The hetero-trimeric Sec protein-conducting channel translocates integral inner membrane proteins and secretory proteins into or across the membrane. The SecYEG core-translocon forms a central pore through which hydrophilic polypeptides are transported, otherwise closed by a girdle of hydrophobic residues and a short helix (plug)8. YidC is required to facilitate this passage from the lateral gate and for the subsequent folding and assembly of inner membrane-proteins and complexes. The ancillary sub-complex comprising SecD and SecF stimulates protein translocation through SecYEG8 assisted by the transmembrane proton-motive force (PMF).

Subsequently, cryo-EM 2D class-averages were aligned against the RCT reconstruction to generate a cryo-EM volume. 3D maximum likelihood refinement using 53,648 particles yielded a low-resolution (14 Å) structure (‘gold-standard’ method and Fourier shell correlation (FSC) criterion 0.14322, Supplementary Fig. S4c,d) with dimensions of 11.4 nm × 10.6 nm × 9.2 nm. Therefore, we placed an E. coli homology model of SecYEG and the E. coli YidC structure as rigid bodies into the respective EM density of the HTL. A homology model of the SecDF sub-complex was placed as a rigid body into the remaining density, with the exception of the SecD P1-domain. Best fit of P1 was achieved independently from the transmembrane part and the SecF periplasmic domain (P4), by rotation of ~120°. The quasi-atomic model corresponding to 75% of HTL was flexibly-fitted into the map employing the molecular dynamics flexible-fitting method and NAMD2.10, coupling the Cα-chain to the map. Importantly, in the HTL the three periplasmic domains of SecD, SecF and YidC adopt a ring-like arrangement, wherein the SecD P1-head and YidC P1 are positioned at the exit site of the SecY translocation channel. Close-by the SecY lateral gate, density attributed to the conserved TM domain of YidC extends to YidC P1-domain. In the inner membrane leaflet, towards the cytoplasmic face of the HTL, there is an inter-connecting density between YidC and SecY, highlighting an interaction. The horseshoe-shape arrangement of the TM-domains of the HTL encloses the central cavity within the protein complex, which is occupied by phospholipids as evidenced by our SANS analyses. We propose that it provides an adaptable, protected environment for membrane-protein insertion, folding and controlled release into the inner membrane.

> MDPSSRDSQRNLLVIALLFVSFMIWQAWEQDKNPQPQAQQTTQTTTTAAGSAADQGVPASGQGKLISVKTDVLDLTINTRGGDVEQALLPAYPKELNSTQPFQLLETSPQFIYQAQSGLTGRDGPDNPANGPRPLYNVEKDAYVLAEGQNELQVPMTYTDAAGNTFTKTFVLKRGDYAVNVNYNVQNAGEKPLEISSFGQLKQSITLPPHLDTGSSNFALHTFRGAAYSTPDAAYAAYAFDTIADNENLNISSKGGWVAMLQQYFATAWIPHNDGTNNFYTANLGNGIAAIGYKSQPVLVQPGQTGAMNSTLWVGPEIQDKMAAVAPHLDLTVDYGWLWFISQPLFKLLKWIHSFVGNWGFSIIIITFIVRGIMYPLTKAQYTSMAKMRMLQPKIQAMRERLGDDKQRISQEMMALYKAEKVNPLGGCFPLLIQMPIFLALYYMLMGSVELRQAPFALWIHDLSAQDPYYILPILMGVTMFFIQKMSPTTVTDPMQQKIMTFMPVIFTVFFLWFPSGLVLYYIVSNLVTIIQQQLIYRGLEKRGLHSREKKKSHHHHHH;> MHHHHHHMLNRYPLWKYVMLIVVIVIGLLYALPNLFGEDPAVQITGARGVAASEQTLIQVQKTLQEEKITAKSVALEEGAILARFDSTDTQLRAREALMGVMGDKYVVALNLAPATPRWLAAIHAEPMKLGLDLRGGVHFLMEVDMDTVLGKLQEQNIDSLRSDLREKGIPYTTVRKENNYGLSITFRDAKARDEAIAYLSKRHPDLVISSQGSNQLRAVMSDARLSEAREYAVQQNINILRNRVNQLGVAEPVVQRQGADRIVVELPGIQDTARAKEILGATATLEFRLVNTNVDQAAAASGRVPGDSEVKQTREGQPVVLYKRVILTGDHITDSTSSQDEYNQPQVNISLDSAGGNIMSNFTKDNIGKPMATLFVEYKDSGKKDANGRAVLVKQEEVINIANIQSRLGNSFRITGINNPNEARQLSLLLRAGALIAPIQIVEERTIGPTLGMQNIEQGLEACLAGLLVSILFMIIFYKKFGLIATSALIANLILIVGIMSLLPGATLSMPGIAGIVLTLAVAVDANVLINERIKEELSNGRTVQQAIDEGYRGAFSSIFDANITTLIKVIILYAVGTGAIKGFAITTGIGVATSMFTAIVGTRAIVNLLYGGKRVKKLSI;> MHHHHHHDDDDKAMGANTEAQGSGRGLEAMKWVVVVALLLVAIVGNYLYRDIMLPLRALAVVILIAAAGGVALLTTKGKATVAFAREARTEVRKVIWPTRQETLHTTLIVAAVTAVMSLILWGLDGILVRLVSFITGLRF;> MAQEYTVEQLNHGRKVYDFMRWDYWAFGISGLLLIAAIVIMGVRGFNWGLDFTGGTVIEITLEKPAEIDVMRDALQKAGFEEPMLQNFGSSHDIMVRMPPAEGETGGQVLGSQVLKVINESTNQNAAVKRIEFVGPSVGADLAQTGAMALMAALLSILVYVGFRFEWRLAAGVVIALAHDVIITLGILSLFHIEIDLTIVASLMSVIGYSLNDSIVVSDRIRENFRKIRRGTPYEIFNVSLTQTLHRTLITSGTTLMVILMLYLFGGPVLEGFSLTMLIGVSIGTASSIYVASALALKLGMKREHMLQQKVEKEGADQPSILP;> VGTGWYSGSPGILYHWPEVLRIQELIMYEALLVVFLIVAIGLVGLIMLQQGKGADMGASFGAGASATLFGSSGSGNFMTRMTALLATLFFIISLVLGNINSNKTNKGSEWENLSAPAKTEQTQPAAPAKPTSDIPN;> VWNCERITISHRKQTMAKQPGLDFQSAKGGLGELKRRLLFVIGALIVFRIGSFIPIPGIDAAVLAKLLEQQRGTIIEMFNMFSGGALSRASIFALGIMPYISASIIIQLLTVVHPTLAEIKKEGESGRRKISQYTRYGTLVLAIFQSIGIATGLPNMPGMQGLVINPGFAFYFTAVVSLVTGTMFLMWLGEQITERGIGNGISIIIFAGIVAGLPPAIAHTIEQARQGDLHFLVLLLVAVLVFAVTFFVVFVERGQRRIVVNYAKRQQGRRVYAAQSTHLPLKVNMAGVIPAIFASSIILFPATIASWFGGGTGWNWLTTISLYLQPGQPLYVLLYASAIIFFCFFYTALVFNPRETADNLKKSGAFVPGIRPGEQTAKYIDKVMTRLTLVGALYITFICLIPEFMRDAMKVPFYFGGTSLLIVVVVIMDFMAQVQTLMMSSQYESALKKANLKGYGR>EKIRFCYYRTRKRGHPGEWQGPTQVLWGGDGAIVVKDRGTD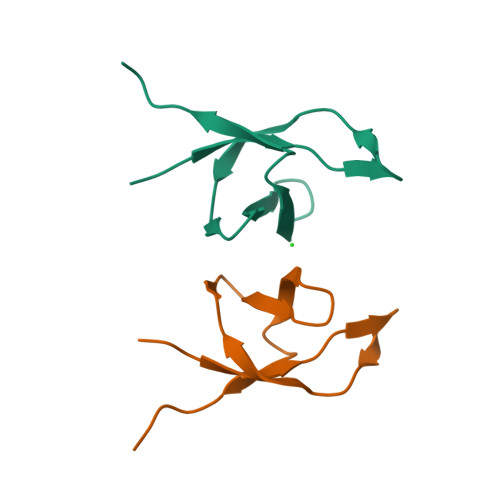RYLVIANKDVKFIPPPK[2x]>GSGNSHTTPWTNPGLAENFMNSFMQGLSSMPGFTASQLDDMSTIAQSMVQSIQSLAAQGRTSPNKLQAL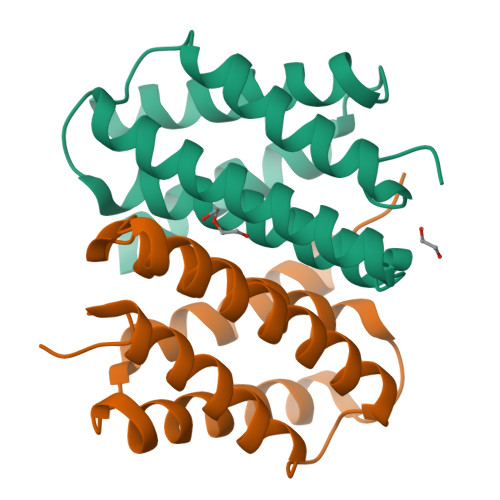NMAFASSMAEIAASEEGGGSLSTKTSSIASAMSNAFLQTTGVVNQPFINEITQLVSMFAQAGMNDVSA[2x]>[4x]MSHGKQFTLYTHKGGPNGWKVTIVLEELGLTYESIFLDFQKGEHKAPEYLKVNPNGRIPALIDHKNNDYTVWESNAIIQYLVDKYDKDRKVSVAPGTNEYYTQLQWLYFQA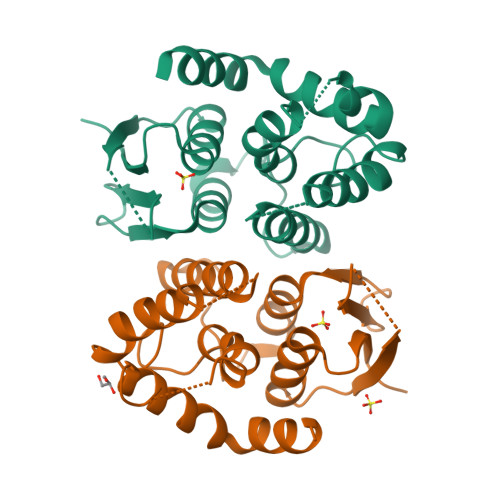SGQGPYYGQAAWFSVYHPEKVPSAIERYRNEIKRVLGVLESVLSKQEFLVDGKATVADFSFLPWNEGAAKFLLEGSQFEEEFPATAKWHKKLLERPAIAKVWEERAKVSAH>[4x]GVWRQYASRALQELGAGKRAIHDVADLTRGSLRIAVTPTFTSYFIGP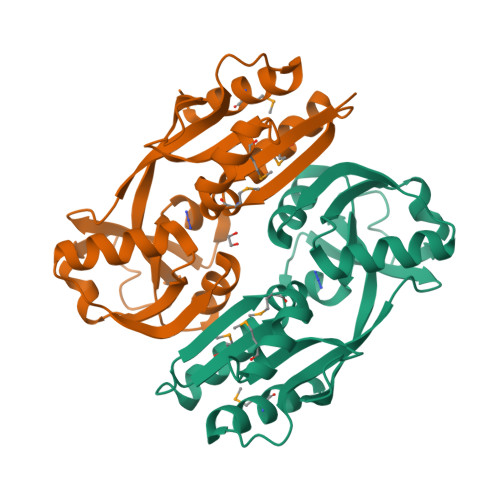LMADFYARYPSITLQLQEMSQEKIEDMLCRDELDVGIAFAPVHSPELEAIPLLTESLALVVAQHHPLAVHEQVALSRLHDEKLVLLSAEFATREQIDHYCEKAGLHPQVVIEANSISAVLELIRRTSLSTLLPAAIATQHDGLKAISLAPPLLERTAVLLRRKNSWQTAAAKAFLHMALDKCAVVGGNESR> MATPDQKSPNVLLQNLCCRILGKSEADVAQQFQYAVRVIGSNFAPTVERDEFLVAEKIKKELTRQRREADAALFSELHRKLHSQGVLKNKWSILYLLLSLSEDPRKQPSKVSGYAALFAQALPRDAH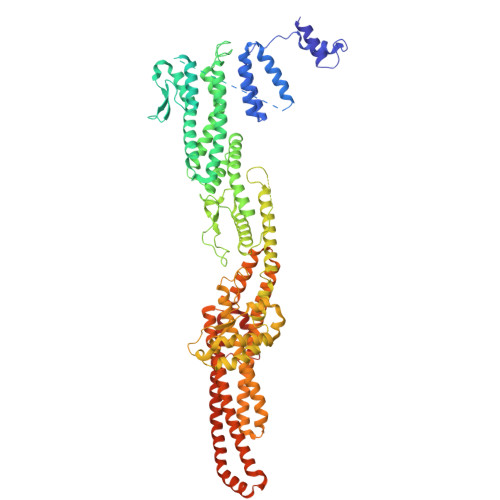STPYYYARPQSLPLNYQERGAPSAQSAGSAGSSGVSSLGTYALNGPTPPPPPPALLPGQPLPAPGVGDGLRQQLGSRLAWTLTASQPSLPSTTSKAVPSSGSRGAARPRREGDAAAGAVEVTEAALVRDILYVFQGIDGKHVKMSNADNCYTVEGKANLSKSLRDTAVRLAELGWLHNKIRKYTDQRSLDRSFGLVGQSFCAALHQELREYYRLLSVLHSQLQLEDDQGVNLGLESSLTLRRLLVWTYDPKMRLKTLAALVDHCQGRKGGELASAVHAYTKTGDPYARSLVQHILSLVSHPVLSFLYRWIYDGELEDTYHEFFVASDPAVKADRLWHDKYALRKPMIPSFMTMDQCRKVLLIGKSINFLHQVCHDQTPTTKMIAVTKSAESPQDAADLFTDLENAFQGKIDAAYFETSKYLLDVLNKKYSLLDHMQAMRRYLLLGQGDFIRHLMDLLKPELVRPATTLYQHNLTGILETAVRATNAQFDSPEILKRLDVRLLEVSPGDTGWDVFSLDYHVDGPIATVFTRECMSHYLRAFNFLWRAKRVEYILTDIRKGHMCNARLLRSMPEFSGVLHHCHILASEMVHFIHQMQYYVTFEVLECSWDELWNRVQRAQDLDHIIAAHEAFLGTVISRCLLDSDSRALLNQLRAVFDQIIELQNTQDAIYRAALEELQRRLQFEEKKKQREAEGQWGVSAAEEEQEKRRVQEFQESIPKMCSQLRILTHFYQGVVQQFLVSLTTSSDESLRFLSFRLDFNEHYRAREPRLRVSLGTRGRRSSHT> ADVPAGVQLADKQTLVRNNGSEVQSLDPHKIEGVPESNVSRDLFEGLLISDVEGHPSPGVAEKWENKDFKVWTFHLRENAKWSDGTPVTAHDFVYSWQRLADPNTASPYASYLQYGHIANIDDI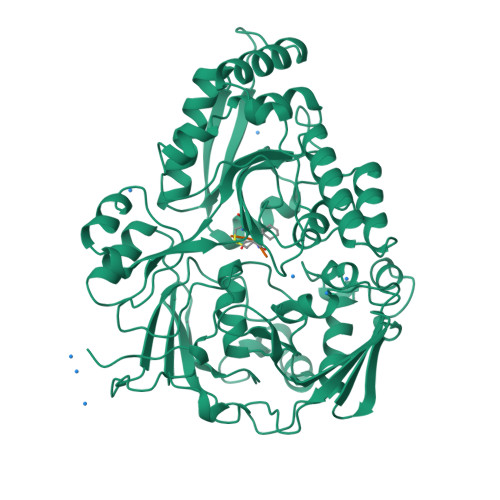IAGKKPATDLGVKALDDHTFEVTLSEPVPYFYKLLVHPSVSPVPKSAVEKFGDKWTQPANIVTNGAYKLKNWVVNERIVLERNPQYWDNAKTVINQVTYLPISSEVTDVNRYRSGEIDMTYNNMPIELFQKLKKEIPNEVRVDPYLCTYYYEINNQKAPFNDVRVRTALKLALDRDIIVNKVKNQGDLPAYSYTPPYTDGAKLVEPEWFKWSQQKRNEEAKKLLAEAGFTADKPLTFDLLYNTSDLHKKLAIAVASIWKKNLGVNVNLENQEWKTFLDTRHQGTFDVARAGWCADYNEPTSFLNTMLSDSSNNTAHYKSPAFDKLIADTLKVADDTQRSELYAKAEQQLDKDSAIVPVYYYVNARLVKPWVGGYTGKDPLDNIYVKNLYIIKH;> KAK> ARKREVRLMKNREAARESRRKKKEYVKCLENRVAVLENQNKTL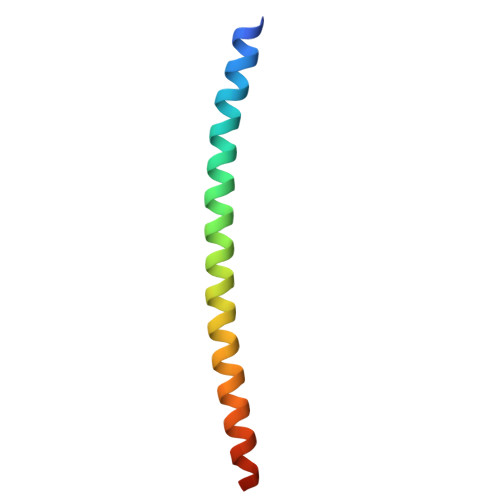IEELKALKDLYSHKSD>SVVLPVAKRGEDILK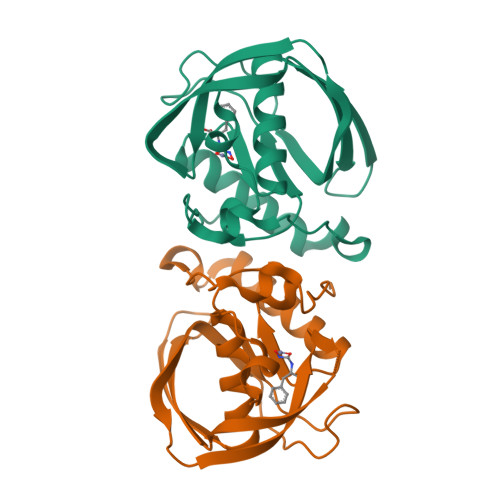LIAAPVSANELNSNWLYQLADAMHATMLERNGVGIAAPQVYISKRVIIVASRPNPRYPDAPEMNAVVMVNPEILEFSSEMCLGEEGCLSVPDERGQVERAEMVKVKYLTLQGEMVETVFQGFPARIVQHEVDHLNGILFVERIS[4x]>[2x]MTMEQFLTSLDMIRSGCA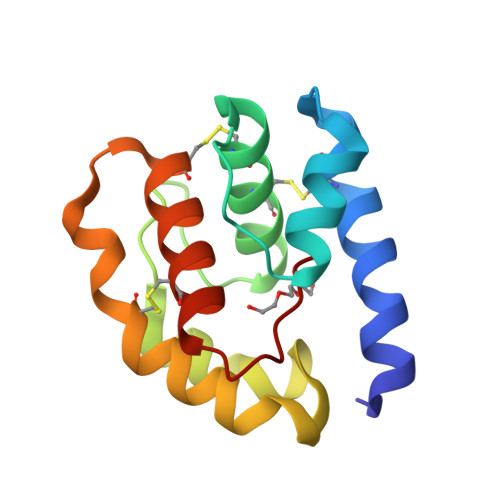PKFKLKTEDLDRLRVGDFNFPPSQDLMCYTKCVSLMAGTVNKKGEFNAPKALAQLPHLVPPEMMEMSRKSVEACRDTHKQFKESCERVYQTAKCFSENAAGQFMWP> SLMEEETHTDAKIRAENGTGSSPRGP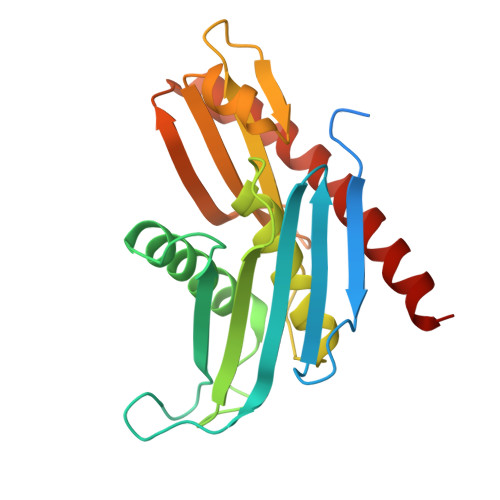GCSLRHFACEQNLLSRPDGSASFLQGDTSVLAGVYGPAEVKVSKEIFNKATLEVILRPKIGLPGVAEKSRERLIRNTCEAVVLGTLHPRTSITVVLQVVSDAGSLLACCLNAACMALVDAGVPMRALFCGVACALDSDGTLVLDPTSKQEKEARAVLTFALDSVERKLLMSSTKGLYSDTELQQCLAAAQAASQHVFRFYRESLQRRYSKS> MPARRPFIGGNFKCNGSLDFIKSHVAAIAAHKIPDSVDVVIAPSAVHLSTAIAANTSKQLRIAAQNVYLEGNGAWTGETSVEMLQDMGLKHVIVGHSERRRIMGETDEQSAKKAKRALEKGMTVIFCVGETLDERKANRTMEVNIAQLEALGKELGESKMLWKEVVIAYEPVWSIGTGVVATPEQAEEVHVGLRKWFAEKVAAEGAQHIRIIYGGSANGSNCEKLGQCPNIDGFLVGGASLKPEFMTMIDILTKTRT

TIM is a ubiquitous glycolytic enzyme whose active site and overall α8/β8 barrel domain structure are highly conserved; even so, structural differences in its interface region have been used to achieve specific inhibition of enzymes in parasites. Since Giardia lacks oxidative phosphorylation and depends on glycolysis as its major ATP source, it has been proposed that disrupting this pathway could hinder the survival of the parasite; therefore, glycolytic enzymes have been considered potential pharmacological targets. Our results indicated that derivatization of C222, a non-interfacial residue located near the surface of the protein and 10-15 Å away from the active site, specifically inactivates the enzyme. C222 is at the end of loop 7, with its lateral chain positioned in a hydrophobic pocket formed mainly by carbon atoms of residues N218, G219, E223, F234, M248, and I251.

WTC, C222NC, C222DC and C222KC rendered crystals suitable for diffraction which, with the exception of C222KC, generated good quality crystallographic data. WTC and C222NC produced high-resolution structures (1.6Å and 1.45Å, respectively), whereas C222DC was solved at a resolution of 2.7Å. In all cases the final maps were of good quality, as indicated by inspection of double difference maps. Remarkably, initial refinement stages yielded immediate interesting results; even though the three proteins were crystallized in presence of 2-PG 5 mM, only the WTC and C222NC structures displayed electronic densities that corresponded to bound ligand in the catalytic site. The structural comparison between WTC and C222NC showed that these structures are almost identical with a Cα RMSD of 0.38 Å2. The larger differences were observed in the region of residues 198-207, which corresponds to a small mobile loop in the middle of helix 6. In both structures the architecture of the catalytic site is conserved; the ligand is positioned correctly and the geometry of the active site residues is preserved. The kinetic and binding data indicated that modification of C222 induces conformational changes that are transmitted as far as 10-15 Å from position 222 to the buried active site (as measured from the sulfur atom of C222 to the 2-PG molecule in the crystal structure of WT GlTIM).>[2x]GSPIGIHMSGQSLTDRITAAQHSVTGSAVSKTVCKATTHEIMGPKKKHLDYLIQCTNEMNVNIPQLADSLFERTTNSSWVVVFKSLITTHHLMVYGNERFI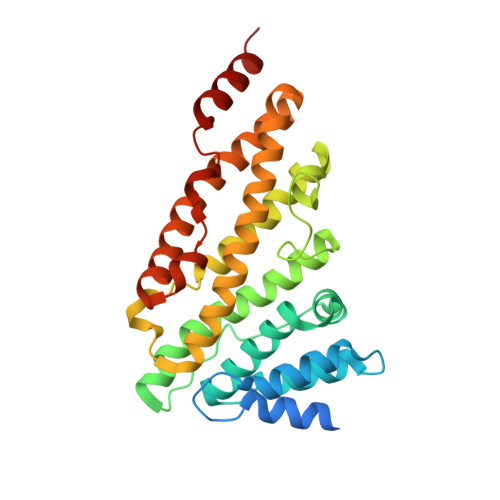QYLASRNTLFNLSNFLDKSGLQGYDMSTFIRRYSRYLNEKAVSYRQVAFDFTKVKRGADGVMRTMNTEKLLKTVPIIQNQMDALLDFNVNSNELTNGVINAAFMLLFKDAIRLFAAYNEGIINLLEKYFDMKKNQCKEGLDIYKKFLTRMTRISEFLKVAEQVGIDRGDIPDLSQAPSSLLDALEQHLASLEGKK> MRGSHHHHHHGSASYEYTSKEELKKTIHAAYLLLDGEFEGIDDSQKDNRVPEVDRTPAEIIAYQLGWLHLVMGWDRDELAGKPVIMPAPGYKWNQLGGLYQSFYAAYADLSLTELRRLFRDTERQWLDWIDTLSEEDLFTQSVRKWTGDKPNWP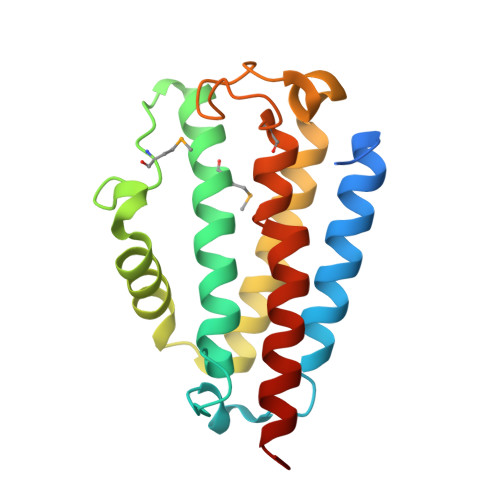MARWIHINSAAPFKTFRAKIRKWKKHQRQA>[2x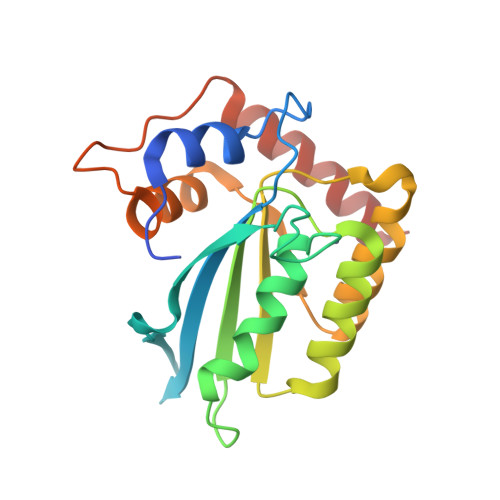]GSHMASLRHSMDPPTFTFNFNNEPWVRGRHETYLCYEVERMHNDTWVLLNQRRGFLCNQAPHKHGFLEGRHAELCFLDVIPFWKLDLDQDYRVTCFTSWSPCFSCAQEMAKFISKNKHVSLCIFTARIYDDQGRCQEGLRTLAEAGAKISIMTYSEFKHCWDTFVDHQGCPFQPWDGLDEHSQDLSGRLRAILQNQEN{hydroxy[(1S)-1-phenylethyl]amino}(oxo)acetic acid | C10 H11 N O4 | 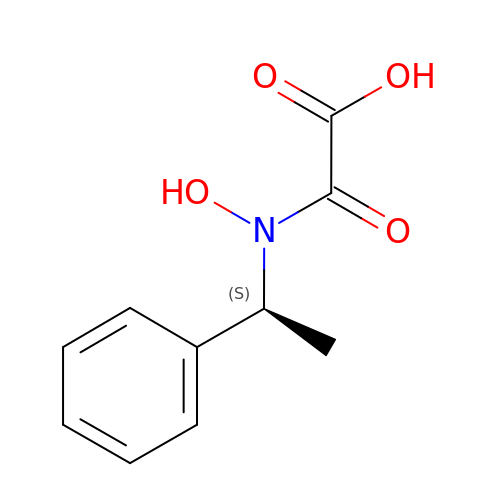IRVSUCQNKPWMLV-ZETCQYMHSA-N~{N}-(3,4-dimethylphenyl)-4-oxidanylidene-chromene-3-carboxamide | 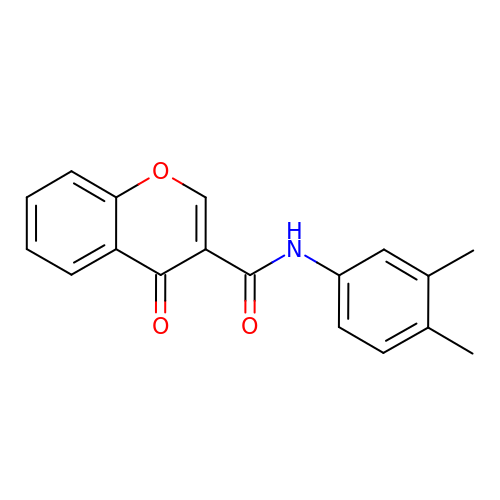C18 H15 N O3 | WDCZOLPCRVTBPH-UHFFFAOYSA-N>QGVQGSAHAINKAGSLRMQSYRLLAAVPLSEKDKPLIKEMEQTAFSAELTRA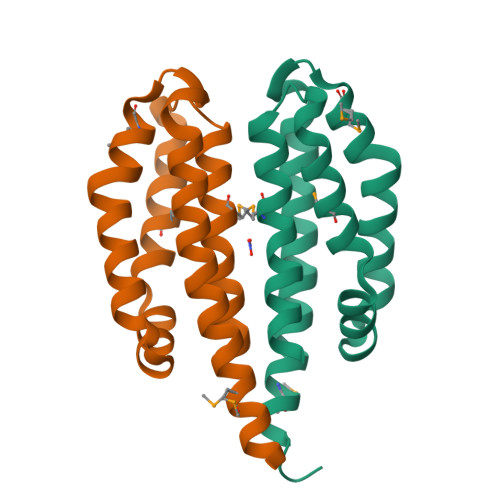AERDGQLAQLQGLQDYWRNELIPALMRAQNRETVSADVSQFVAGLDQLVSGFDRTTEMRIETAAALEHHHHHH[2x]> YNEQYVNKLENFKIRETQGNNGW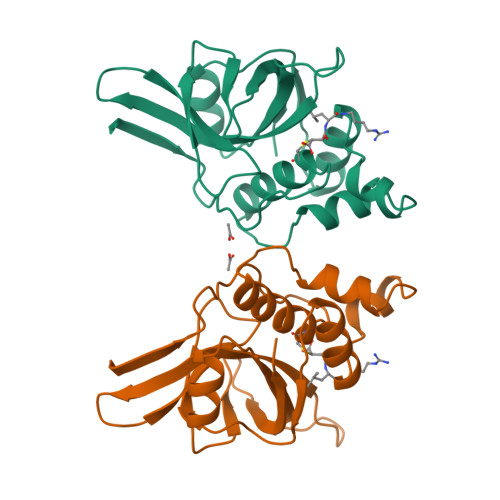CAGYTMSALLNATYNTNKYHAEAVMRFLHPNLQGQQFQFTGLTPREMIYFGQTQGRSPQLLNRMTTYNEVDNLTKNNKGIAILGSRVESRNGMHAGHAMAVVGNAKLNNGQEVIIIWNPWDNGFMTQDAKNNVIPVSNGDHYQWYSSIYGY>[2x]SVDDSKYQCVKLNDGHFMPVLGFGTYAPAEVPKSKALEAVKLAIEAGFHHIDSAHVYNNEEQVGLAIRSKIADGSVKREDIFYTSKLWSNSHRPELVRPALERSLKNLQLDYVDLYLIHFPVSVKPGEEVIPKDENGKILFDTVDLCATWEAMEKCKDAGLAKSIGVSNFNHRLLEMILNKPGLKYKPVCNQVECHPYFNQRKLLDFCKSKDIVLVAYSALGSHREEPWV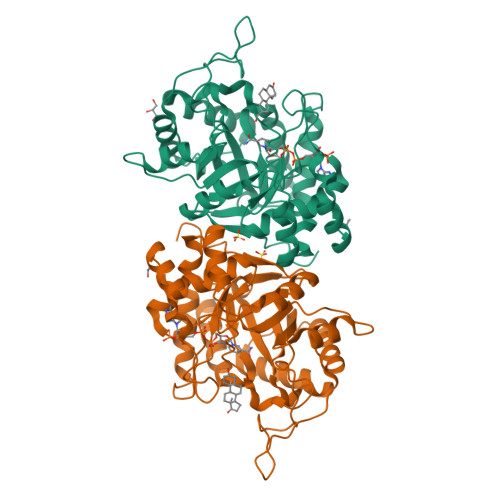DPNSPVLLEDPVLCALAKKHKRTPALIALRYQLQRGVVVLAKSYNEQRIRQNVQVFEFQLTSEEMKAIDGLNRNVRYLTLDIFAGPPNYPFSDEY>[2x]MSATTLTLQQFSTVYNMLSFAVASMLGAFAFFVMGRKIVGPKYRLALVVSSLVVLIAGYHYWRIMGSWTAAYALKDGMYVPTGEPFNDAYRYVDWLLTVPLLLTELVLVMKLKKESGSVLAKLILAAIAMIALGYPGEISNPESQ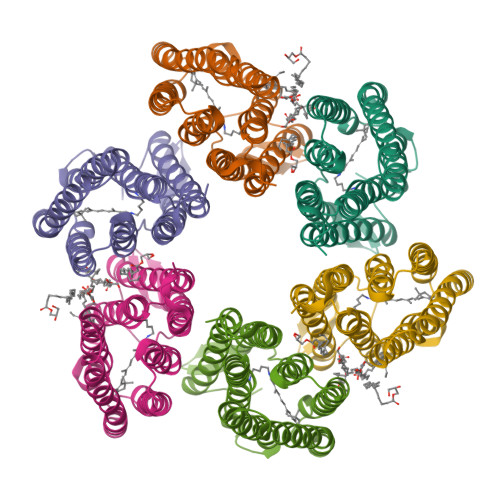AGARLMWGVLSTVPFLYILYVLWVRLGDAIGEHPAKVQVLLKNTRYLILLTWGFYPIVYAMGSYGWLGGAGSVVAVQVGYSIADVTAKALYGVMIFAIAYAKSEADGSLPAHHHHHH2-O-[(R)-{[(2S)-1,1-dihydroxypropan-2-yl]oxy}(hydroxy)phosphoryl]-alpha-D-glucopyranose | C9 H19 O11 P | 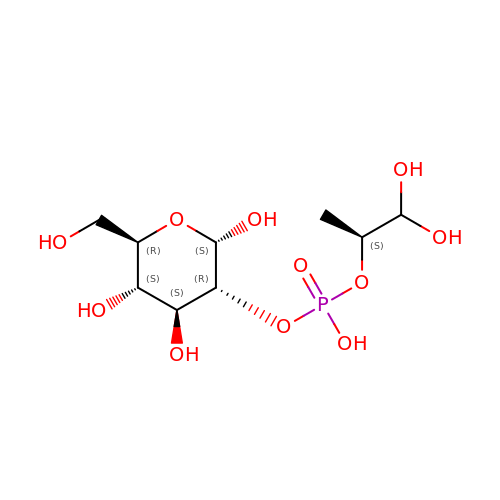SILWFZFNYLTARD-MRXKBSKTSA-N> MILIRNVRLVDARGERGPADVLIGEGRILSLEGGEAKQVVDGTGCFLAPGFLDLHAHLREPGEEVKEDLFSGLLAAVRGGYTDLVSMPNTKPPVDTPEAVRALKEK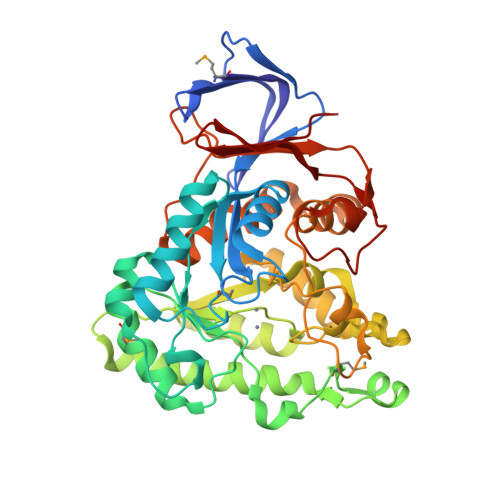AKALGLARLHPAAALTEKQEGKTLTPAGLLREAGAVLLTDDGRTNEDAGVLAAGLLMAAPLGLPVAVHAEDAGLRRNGVMNDGPLADLLGLPGNPPEAEAARIARDLEVLRYALRRSPATPRLHVQHLSTKRGLELVREAKRAGLPVTAEATPHHLTLTEEALRTFDPLFKVAPPLRGEEDREALLEGLLDGTLDAIATDHAPHTLAEKEKDLLRAPFGIPSLEVAFPLLYTELHLKRGFPLQRLVELFTDGPRRVLGLPPLHLEEGAEASLVLLSPKERPVDPSAFASKARYSPWAGWVLGGWPVLTLVAGRIVHEALK> MDYKDDDDKDYK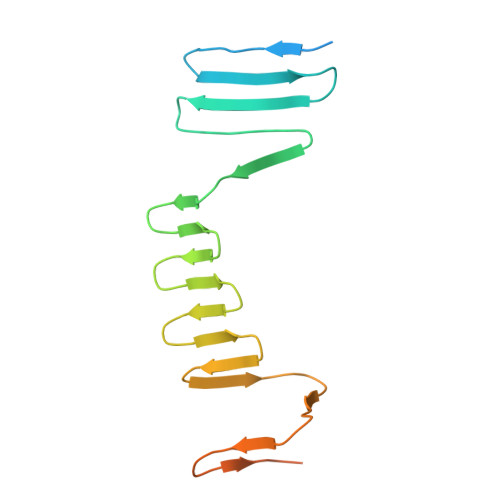DDDDKDYKDDDDKGSKADHIFNLEEQGLLIDIKDDSKGCTTKLESSGKITHNATESIESSADKQIIENVKDSKISITEKEILLATKKSSIMLSEDKIVIKIGNSLIILDDSNISLESATINIKSSANINIQASQNIDIKSLNNSIKADVNLNAEGLDVNIKGSVTASIKGSAATMVG> CLAEGTRIFDPVTGTT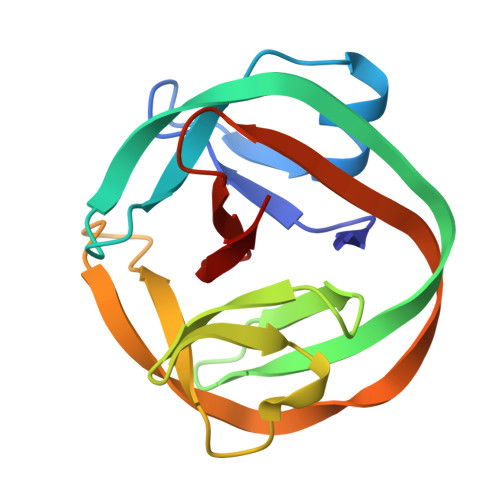HRIEDVVDGRKPIHVVAAAKDGTLHARPVVSWFDQGTRDVIGLRIAGGAILWATPDHKVLTEYGWRAAGELRKGDRVAVRDVETGELRYSVIREVLPTRRARTFDLEVEELHTLVAEGVVVHN> APTMPPP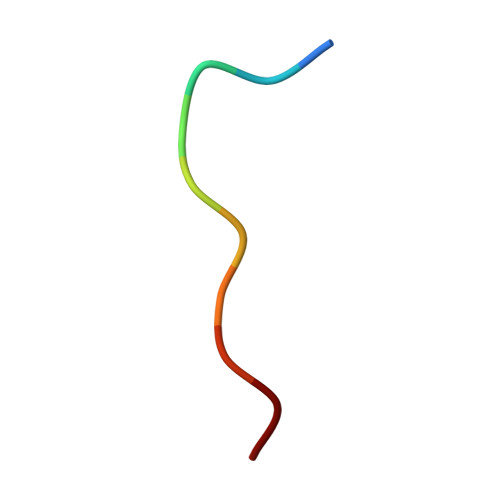LPP> MAHHHHHHSAALEVLFQGPGPAASSNHWQIPELARKVNTEQKHTTFEQPVFSVSKQSPPISTSKWFDPKSICKTPSSNTLDDYMSCFRTPVVKNDFPPACQLSTPYGQPACFQQQQHQILATPLQNLQVLASSSANECISVKGRIYSILKQIGSGGSSKVFQVLNEKKQIYAIKYVNLEEADNQTLDSYRNEIAYLNKLQQHSDKIIRLYDYEITDQYIYMVMECGNIDLNSWLKKKKSIDPWERKSYWKNMLEAVHTIHQHGIVHSDLKPANFLIVDGMLKLIDFGIANQMQPDTTSVVKDSQVGTVNYMPPEAIKDMSSSRENGKSKSKISPKSDVWSLGCILYYMTYGKTPFQQIINQISKLHAIIDPNHEIEFPDIPEKDLQDVLKC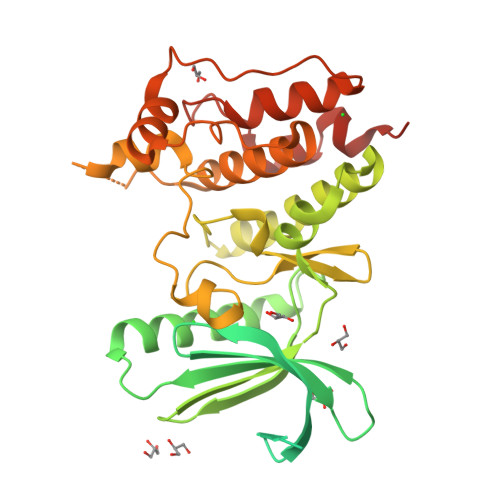CLKRDPKQRISIPELLAHPYVQIQTHPVNQMAKGTTEE> SARLETVQADNIREKKEKLALRQQLNEAKQQLLQQAEYCTEMGAAACTLLWGVSSSEEVVKAILGGDKALKFFSITGQTMESFVKSLDGDVQELDSDESQFV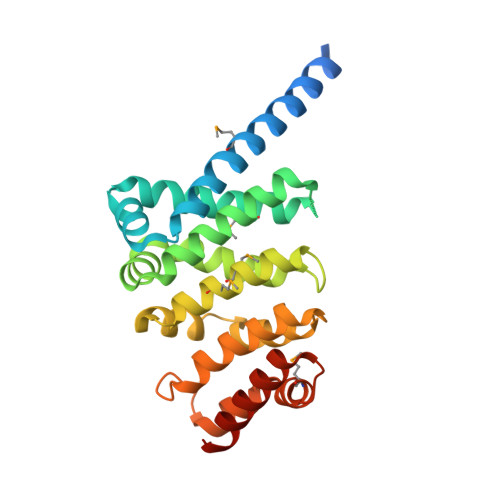FALAGIVTNVAAIACGREFLVNSSRVLLDTILQLLGDLKPGQCTKLKVLMLMSLYNVSINLKGLKYISESPGFIPLLWWLLSDPDAEVCLHVLRLVQSVVLEPEVFSKSASEFRSSLPLQRILAMSKSRNPRLQTAAQELLEDLRTLEHNV>MPQGPEVALTADILEKYFKGKTLEYIDFISGRYSKSEPEGYDDFIANLPLKVSNVDTKGKFLWFELFDPNDKSNKWYIWNTFGLTGMWSLFEAKYTRAVLSFDNELMAYFSDMRNFGTFKFSNSEKELKRKLNELGPDFLKNDDIDISKIKKYKQPIVALLMDQKKIGSGLGNYLVAEILYRAKIDPHKLGSNLTDQEIENLWYWIKYETKLAYDSNHIGYMVNLENESSKIGRKNYHPNIHPTEKEFDFLVYRKKKDPNGNKVIADKIIGSGK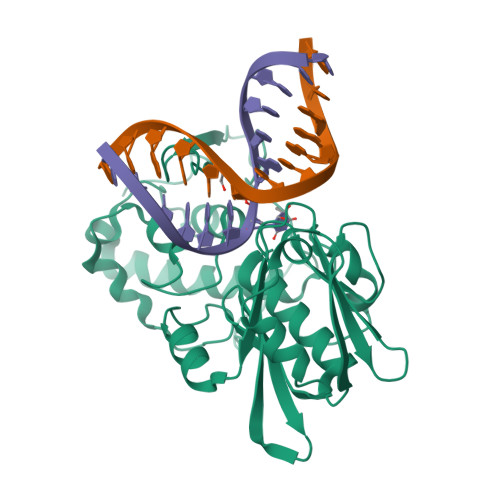NKRTTYWAPAIQKLEHHHHHH[2x]> DH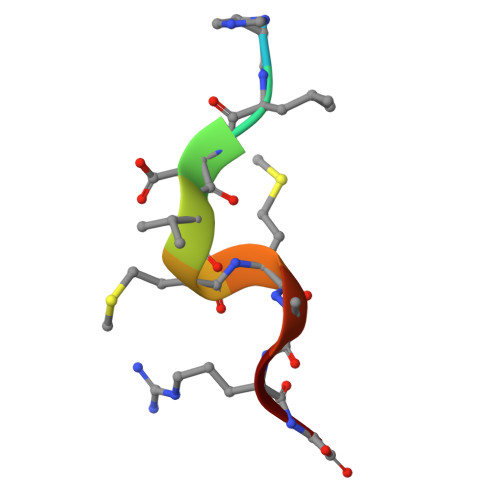LDVMMARG>KDMFNTKSSNGKLRIEDASHNARKLGLAPSSTDEKKIRDLYGD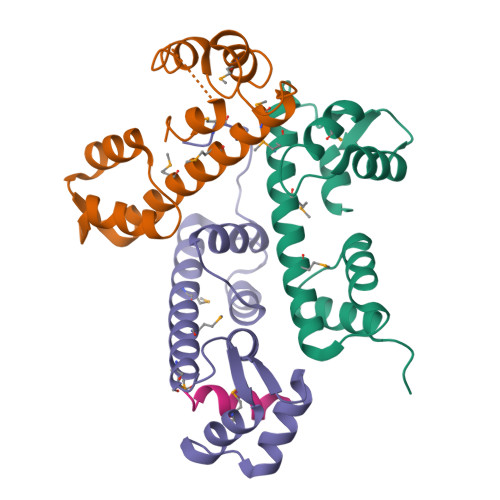SLTYEQYLEYLTMCVHDRDNMEELIKMFSHFDNNSSGFLTKNQMKNILTTWGDALTEQEANDALNAFSSEDRINYKLFCEDIL[3x];> SLMRVQAHIRKRMVA>GMNIDEIERKIDEAIEKEDYETLLSLLNKRKELMEGLPKDKLSEILEKDRKRLEIIEKRKTALFQEIN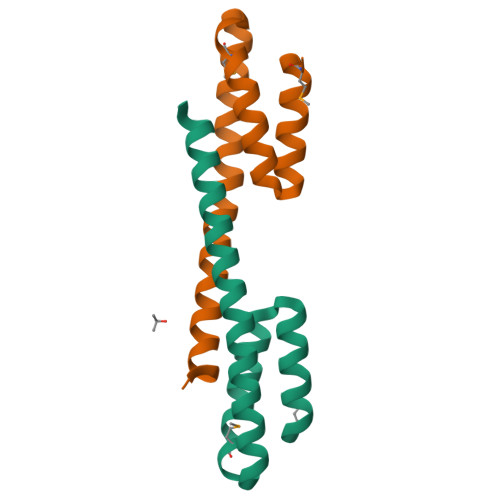VIREARSSLQK[2x]>DEAKISAQSFYQRLLLLNEEAILSGQDFGVRIDVDTRRLTFLQLTADKGWQKWQNDKMTNQTTLKEGLQLDFELGGGAWQKDDRLFNPGSLFDEEMFADEKKEQKQEPAPQLFVL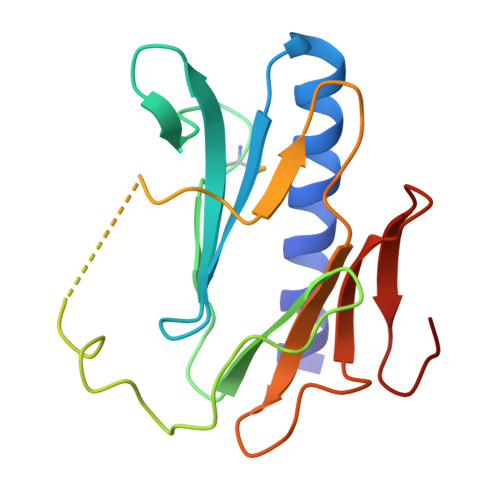SSGEVTPFTLSIFPKGQEPDEQWRVTAQENGTLRLLAPGESDEE[2x]> MKHHHHHHMKQNSPLDEENLTQENQDRGTHVDRGLASANVDFAFSLYKQLVLKAPDKNVIFSPLSISTALAFLSLGAHNTTLTEILKGLKFNLTETSEAEIHQSFQHLLRTLNQSSDELQLSMGNAMFVKEQLSLLDRFTEDAKRLYGSEAFATDFQDSAAAKKLINDYVKNGTRGKITDLIKDLDSQTMMVLVNYIFFKAKFEMPFDPQDTHQSRFYLSKKKYVMVPMMSLHHLTIPYFRDEELSCTVVQLNY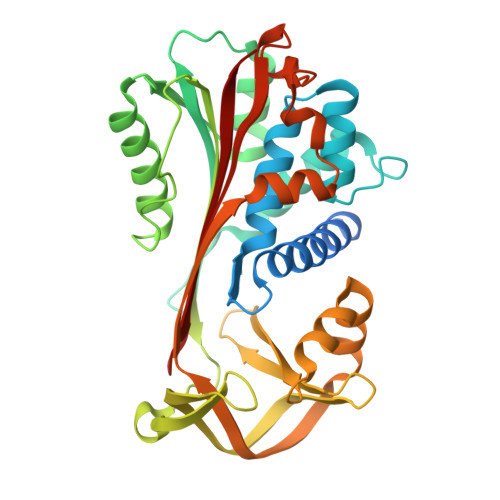TGNASALFILPDQDKMEEVEAMLSQETLSRFFESLEFREIGELYLPKFSISRDYNLNDILLQLGIEEAFTSKADLSGITGARNLAVSQVVHKAVLDVFEEGTEASAATALEVLFQ>[2x]GSHGQYLLPEAKAQDSDKICVVIDLAETLVHSSFKPVNNADFIIPVE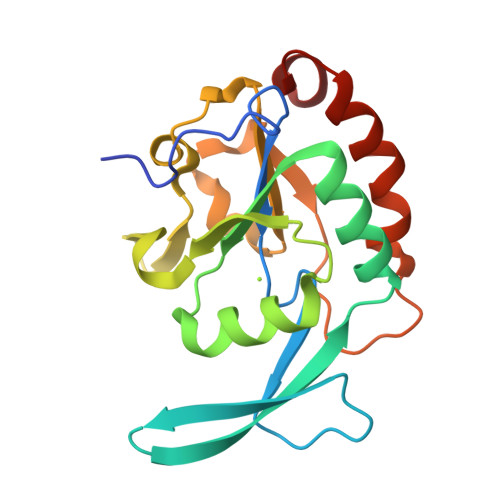IDGVVHQVYVLKRPHVDEFLQRMGELFECVLFTASLAKYADPVADLLDKWGAFRARLFRESCVFHRGNYVKDLSRLGRDLRRVLILDNSPASYVFHPDNAVPVASWFDNMSDTELHDLLPFFEQLSRVDDVYSVLRQ>MATEVTFFDELKIDNKVDIIGNNVRGELPNIWLQYGQFKLKASGGDGTYSWYSENTSIATVDASGKVTLNGKGSVVIKATSGDKQTVSYTIKAPSYMIKVDKQAYYADAMSICKNLLPSTQTVLSDIYDSWGAANKYSHYSSMNSITAWIKQTSSEQRSGVSSTYNLITQNPLPGVNVNTPNVYAVCVE[4x]

Intimin, an out membrane protein expressed by EHEC and EPEC, is required for intimate attachment to the host cell and formation of the A/E lesions. The binding of intimin to Tir mediates the adhesion between the pathogen and its host cell. The intimin of EHEC O157:H7 is of γ-type (designated intimin-γ), whereas that of EPEC is intimin-α. Here, we determined the crystal structures of Tir-binding domain of EHEC O157:H7 intimin at 2.8 Å, together with an Asn to Tyr mutant at amino acid 916 (IntN916Y) at 2.6 Å.

Crystals of EHEC Int188 and IntN916Y diffract X-rays at 2.8 Å and 2.6 Å, respectively. R-free values were separately refined to 29.6% and 26.8%. These two versions of intimin (Int188 and IntN916Y) were crystallized in space group C2 and P212121, respectively. For the native version, Int188 consists of four molecules in the asymmetric unit while the IntN916Y is present in two molecules per asymmetric unit. Topological analysis suggest that Int188 is composed of sixteen beta-sheets together with four alpha-helices, which can be supported by the crystal structure. Both topological and structural evidence indicate that Int188 can be obviously categorized into two independent domains (Domain I& Domain II). Further structural blast revealed that these two domains correspond to an Ig-like domain and a C-type lectin-like domain, respectively. The Ig-like domain at the N-terminus of Int188 is composed of beta-sheet sandwiches which contain eleven anti-parallel beta-sheets (A, A′, A″, A″′, B, B′, C, D, E, F and G) and ten coils. Beta-sheets A′ and A″ between strands A and A′″ extend a platform on top of Domain I that contacts Domain II, helping to define the relative orientation of the two domains. A C-type lectin-like domain was found to be located at its C-terminus, comprised of two anti-parallel beta-sheets (B, C, D and A, E) spaced by four alpha-helices (I, II, III and IV). C932 in the C-terminal strand E forms a disulfide bond with the C858 in helix I. Strand E and strand A in N-terminus of Domain II form the principal strands of the first sheet. BLAST analysis reveals that although EHEC Int188 is of 48% sequence identity to that of EPEC, the secondary structures of both proteins are similar in the topological characterization.>QKQLRGQIARRVYRQLLAEKRAEEEKRKREEEEKRKREEEERERERERREAELRAQQEEAARKQRELEA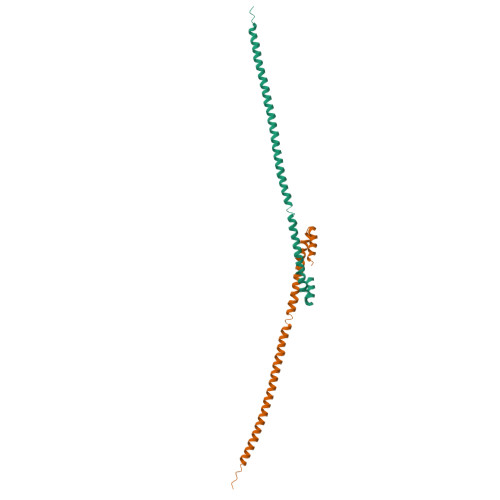LQQESQRAAELSRELEKQKENKQVEEILRLEKEIEDLQRMKERQELSLTEASLQKLQQLRDEELR[2x]> GQAFRKFLPLFDRVLVERSAAETVTKGGIM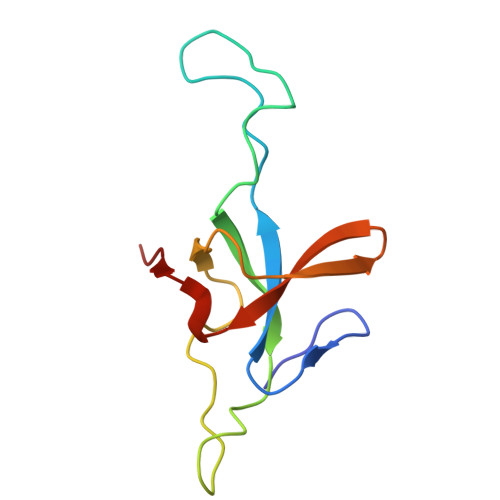LPEKSQGKVLQATVVAVGSGSKGKGGEIQPVSVKVGDKVLLPEYGGTKVVLDDKDYFLFRDGDILGKYVD> LADGAHIGNYQIVKTLGEGSFGKVKLAYHTTTGQKVALKIINKKVLAKSDMQGRIEREISYLRLLRHPHIIKLYDVIKSKDEIIMVIEYAGNELFDYIVQRDKMSEQEARR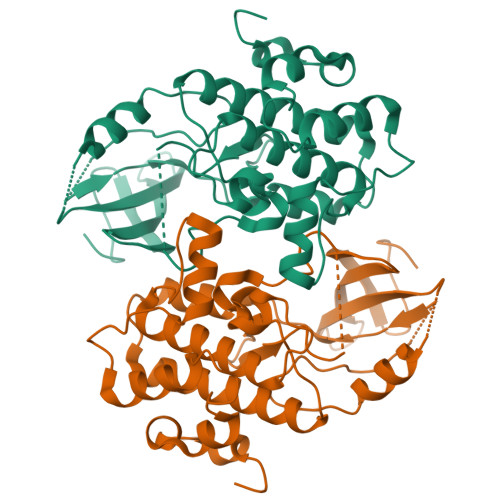FFQQIISAVEYCHRHKIVHRDLKPENLLLDEHLNVKIADFGLSNIMTDGNFLKTSCGSPNYAAPEVISGKLYAGPEVDVWSCGVILYVMLCRRLPFDDESIPVLFKNISNGVYTLPKFLSPGAAGLIKRMLIVNPLNRISIHEIMQDDWFKVDLPEYLLPPDL>MPTLLRVYIDGPHGMGKTTTTQLLVALGSRDDIVYVPEPMTYWRVLGASETIANIYTTQHRLDQGEISAGDAAVVMTSANITMGMPYAVTDAVLAPHIGGEAGSSHAPPPALTLIFDRHPIAALLCYPAARYLMGSMTPQAVLAFVALIPPTLPGTNIVLGALPEDRHIDRLAKRQRPGERLDLAMLAAIRRVYGLLANTVRYLQCGGSWREDWGQLSGTAVPPQGAEPQSNAGPRPHIGDTLFTLFRAPELLAPNGDLYNVFAWALDVLAKRLRSMHVFILDYDQSPAGCRDALLQLTSGMVQTHVTTPGSIPTICDLARTFAREMGE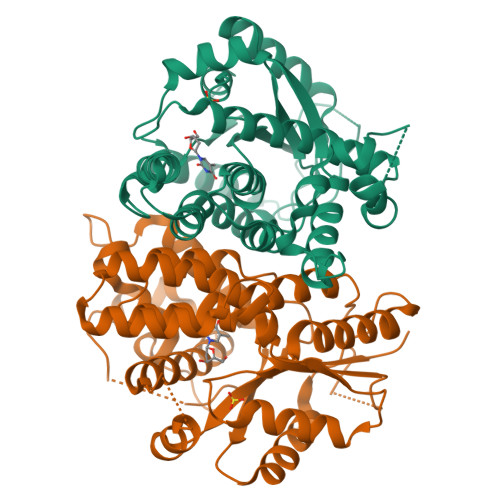AN[2x]> MKDLLKFLKAQTKTEEFDAIKIALASPDMIRSWSFGEVKKPETINYRTFKPERDGLFCARIFGPVKDYECLCGKYKRLKHRGVICEKCGVEVTQTKVRRERMGHIELASPTAHIWFLKSLPSRIGLLLDMPLRDIERVLYFESYVVIEGGMTNLERQQILTEEQYLDALEEFGDEFDAKMGAEAIQALLKSMDLEQECEQLREELNETNSETKRKKLTKRIKLLEAFVQSGNKPEWMILTVLPVLPPDLRPLVPLDGGRFATSDLNDLYRRVINRNNRLKRLLDLAAPDIIVRNEKRMLQEAVDALLDNGRRGRAITGSNKRPLKSLADMIKGKQGRFRQNLLGKRVDYSGRSVITVGPYLRLHQCGLPKKMALELFKPFIYGKLELRGLATTIKAAKKMVEREEAVVWDILDEVIREHPVLLNRAPTLHRLGIQAFEPVLIEGKAIQLHPLVCAAYNADFDGDQMAVHVPLTLEAQLEARALMMSTNNILSPANGEPIIVPSQDVVLGLYYMTRDCVNAKGEGMVLTGPKEAERLYRSGLASLHARVKVRITEYEKDANGELVAKTSLKDTTVGRAILWMIVPKGLPYSIVNQALGKKAISKMLNTCYRILGLKPTVIFADQIMYTGFAYAARSGASVGIDDMVIPEKKHEIISEAEAEVAEIQEQFQSGLVTAGERYNKVIDIWAAANDRVSKAMMDNLQTETVINRDGQEEKQVSFNSIYMMADSGARGSAAQIRQLAGMRGLMAKPDGSIIETPITANFREGLNVLQYFISTHGARKGLADTALKTANSGYLTRRLVDVAQDLVVTEDDCGTHEGIMMTPVIEGGDVKEPLRDRVLGRVTAEDVLKPGTADILVPRNTLLHEQWCDLLEENSVDAVKVRSVVSCDTDFGVCAHCYGRDLARGHIINKGEAIGVIAAQSIGEPGTQLTMRTFHIGGAASRAAAESSIQVKNKGSIKLSNVKSVVNSSGKLVITSRNTELKLIDEFGRTKESYKVPYGAVLAKGDGEQVAGGETVANWDPHTMPVITEVSGFVRFTDMIDGQTITRQTDELTGLSSLVVLDSAERTAGGKDLRPALKIVDAQGNDVLIPGTDMPAQYFLPGKAIVQLEDGVQISSGDTLARIPQESGGTKDITGGLPRVADLFEARRPKEPAILAEISGIVSFGKETKGKRRLVITPVDGSDPYEEMIPKWRQLNVFEGERVERGDVISDGPEAPHDILRLRGVHAVTRYIVNEVQDVYRLQGVKINDKHIEVIVRQMLRKATIVNAGSSDFLEGEQVEYSRVKIANRELEANGKVGATYSR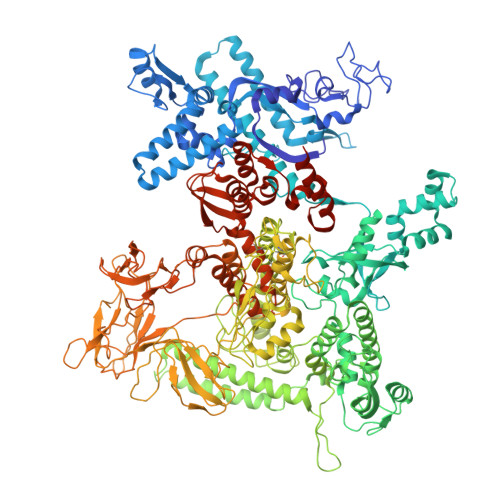DLLGITKASLATESFISAASFQETTRVLTEAAVAGKRDELRGLKENVIVGRLIPAGTGYAYHQDRMRRRAAGEAPAAPQVTAEDASASLAELLNAGLGGSDNE>MAHHHHHHTSTLMGSLTMLGKAGCQWEHANTSFASFSNVVACNTATVTGLASAPTEGKIPGIRFANLPAGDYELTVLIFSMYPVDAGVYCRYRLWDGTNF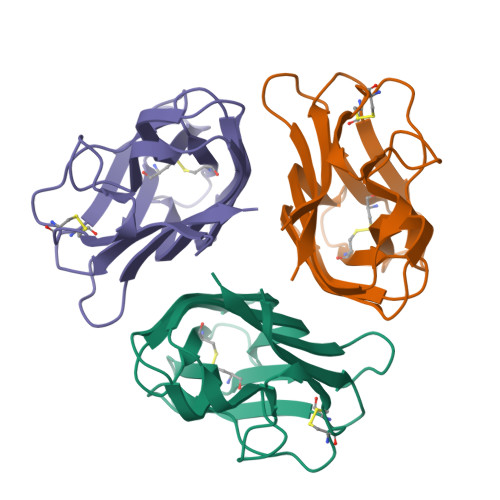SGMAGAYESEIYQMTGLFSYATDQTNLTFYVQAQTLTATKNCRADITVPGQDKMQIYLKKL[3x]>KQVENYDSWEDLVSSIDTIERKDDGTLEIYLTWKNGAISHHPSTITNKKCPQKMLQFYESHLTFRENE[2x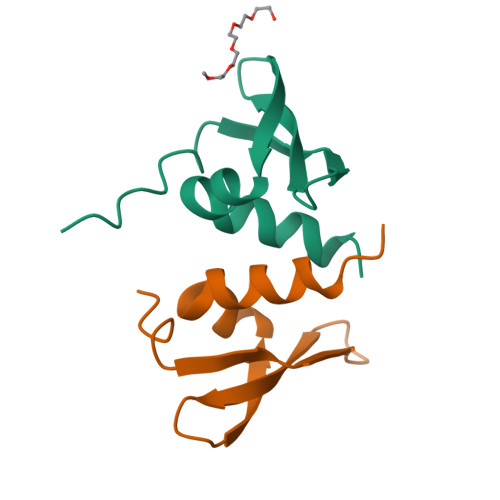]>[2x]SNAMLLYTKKDDIYSDIVRMILLIKGANAKIVDVSKEENSKHLEELNIITPNGNIPTLSTDDFAVYRLSVIIEAIEDLYPFPPMFPVFPKQRANARILLEYVNKTFLQNIIKLQSPDLDEKQANEIKMLMQRDIISTYKKIVSEREVNAESNPDAQNINVLTLIITFVFYYFIKLKISIPTKDKNIIKEIKELLSEPNFIKTIK;>[2x]SNAMVTLYTTKYCPYSLRARIALAEKKMSTDIVEAGDLEPAMIKKITPNGVFPVLMEKDYSINNRKALLIYIDERFPAPSLLPNVVNERIKIRLSLDKIDNEWYPVLDQIRKHRSDQKMLESMFKDLKESLLAMEKAFTGSEFFISSGFTLADCYIAALIICLEAEGFIIDDEYGAIYEYKKRLFARDSVKKANIKGGAGESLLKTLRTHR

An unusual set of Francisella regulators—the heteromeric macrophage growth locus protein A (MglA)–stringent starvation protein A (SspA) complex and the DNA-binding protein pathogenicity island gene regulator (PigR)—activates FPI transcription and thus is essential for virulence. The F. tularensis SspA protein, which shares ∼30% sequence identify with other bacterial SspAs, is not homodimeric and instead forms a complex with MglA. Multiple studies have shown that SspA proteins impart their function through interaction with RNA polymerase (RNAP), and, in Francisella, both MglA and SspA are required for RNAP interaction. Here we identify MglA–SspA as a novel ppGpp-binding complex and describe structures of apo- and ppGpp-bound MglA–SspA.

The structure was solved to 2.8 Å resolution and refined to final Rwork/Rfree values of 21.2%/26.5%. In each dimer, clear electron density was observed for a single ppGpp–Mg2+ molecule that, strikingly, binds in the open face of the heterodimer with a stoichiometry of one ppGpp to one MglA–SspA dimer. Comparison of the apo- and ppGpp-bound MglA–SspA structures showed that the individual subunits and the heterodimer did not undergo any large structural changes upon ppGpp binding (superimposition of the apo- and ppGpp-bound heterodimers gives RMSDs of 0.7–0.8 Å). The majority of the interactions to the ppGpp in the MglA–SspA–ppGpp structure is provided by MglA. The ppGpp in the (MglA–SspA)–ppGpp complex adopts a ring-like conformation, which is stabilized by a bound Mg2+. Binding of the Mg2+ to the phosphates is crucial for stabilizing the bound ring-like structure, which assumes a conformation optimal for docking in the MglA–SspA-binding pocket. The backbone amide group of MglA residue Leu65 and the carbonyl oxygen moiety of MglA residue Ile52 play key roles in guanine base recognition by making hydrogen bonds to the O6 and N7 atoms, respectively. Aside from the base-specific interactions with the guanine, additional hydrophilic and hydrophobic contacts anchor the ppGpp molecule into the binding pocket. These contacts include stacking interactions between MglA residue Tyr11 and the guanine base as well as ribose hydroxyl interactions from MglA residues Asn100 and Gln105. The ppGpp pyrophosphate moieties are contacted by the side chains of MglA residues Arg64 and Lys101. Intriguingly, SspA makes only two interactions with the bound ppGpp-Mg2+: one from residue Lys65 to the ppGpp phosphate groups and another from residue Asn100, which interacts with the Mg2+ ion.> MTISRVKLLDTMVDTFLQKLVAAGSYQRFTDCYKCFYQLQPAMTQQIYDKFIAQLQTSIREEISDIKEEGNLEAVLN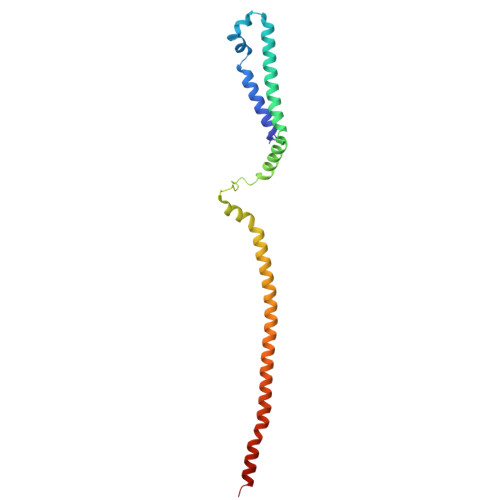ALDKIVEEGKVRKEPAWRPSGIPEKDLHSVMAPYFLQQRDTLRRHVQKQEAENQQLADAVLAGRRQVEELQLQVQAQQQAWQALHREQRELVAVLREPE>[4x]QALSEIETRHSEIIKL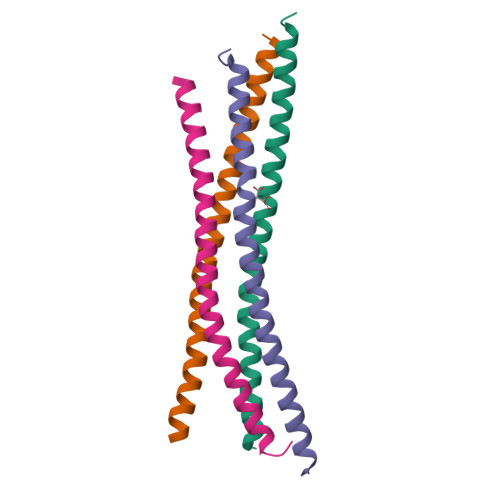ENSIRELHDMFMDMAMLVESQGEMIDRIEYNVEHAVDYVERAVSDTKKAVKYQSKARRK> GYLVGDATRGANLWNTQTCVACHGVDGERNASGTPALTPLNPNRDLYRHSRDTQDRALRDFISMWMPQGNEGSCTGQCAADIEAFIRTWHHHHHH

Here we analyse a small c-type cytochrome (CjX183) present in Cellvibrio japonicus Cbp2D, and show that it can initiate bacterial CuII/I LPMO reduction and also activate LPMO-catalyzed cellulose-degradation. Gardner et al. have shown previously that cbp2D codes for a protein that is predicted to contain a carbohydrate-binding module, a YceI-like quinone binding domain, a fibronectin type III (FN3) domain and two c-type cytochrome domains. Here, we present the structure of a domain from Cbp2D, which we dub CjX183, confirming that it is indeed a small c-type cytochrome domain, with an exposed heme cofactor. Here, we have determined the structure of the isolated X183 domain (CjX183) from this protein, confirming it as a typical c-type cytochrome that most likely has an electron transferring (rather than a catalytic) function.

CjX183 was expressed in the periplasm of E. coli with the aid of the pEC86 vector which codes for the cytochrome maturation machinery to allow the insertion of heme into the protein. The red coloured protein was subsequently purified to homogeneity, crystallized and the structure determined to 1.2 Å resolution (see Supplementary Table S1 for structure solution and refinement statistics). The structure reveals CjX183 to be an α-helical c-type cytochrome domain harbouring a single heme molecule, which is covalently linked to the conserved CXXCH motif via thioether linkages to Cys19 and Cys22. Two additional cysteines (residues 74 and 78) are present towards the C-terminus of the domain and these form a disulfide bond, presumably to stabilise the protein in the extracellular environment. The central heme iron atom is coordinated by a proximal histidine residue, His23, and a distal methionine residue, Met66 in the typical configuration observed for class one c-type cytochromes. Interestingly, the edges of the heme molecule appear to be largely solvent exposed, however, the propionate groups form hydrogen bonds with Arg44 and Ser50 located in a surface loop which extends around this part of the molecule. These interactions may account for the relative stability of the reduced state discussed later. CjX183 aligns to the electron transfer domain within TsdA, suggesting a similar electron transfer role for CjX183 as is typical of this cytochrome class. Analysis of these signals indicates that they arise from a one-electron redox reaction that is attributed to the reversible FeIII/II chemistry of the heme within CjX183. This experiment suggested that in principle CjX183 is capable of activating LPMOs because the extracted midpoint potential (+193 mV vs SHE) sits below the reduction potentials that have been reported for LPMOs (typically greater than +220 mV vs SHE). The complete oxidation of the heme in CjX183 took ∼2 h demonstrating that it remains reduced in the presence of O2 for an extended period, even though the structure reveals that the heme is quite solvent exposed.>SMAAATFHWDDPLLLDQQLADDERMVRDAAHAYAQGKLAPRVTEAFRHETTDAAIFREMGEIGLLGPTIPEQYGGPGLDYVSYGLIAREVERVDSGYRSMMSVQSSLVMVPIFEFGSDAQKEKYLPKLATGEWIGCFGLTEPNHGSDPGSMVTRARKVPGGYSLSGSKMWITNSPIADVFVVWAKLDEDGRDEIRGFILEKGCKGLSAPAIHGKVGLRASITGEIVLDEAFVPEENILPHVKGLRGPFTCLNSARYGIAWGALGAAESCWHIARQYVLDRKQFGRPLAANQLIQKKLADMQTEITLGLQGVLRLGRMKDEGTA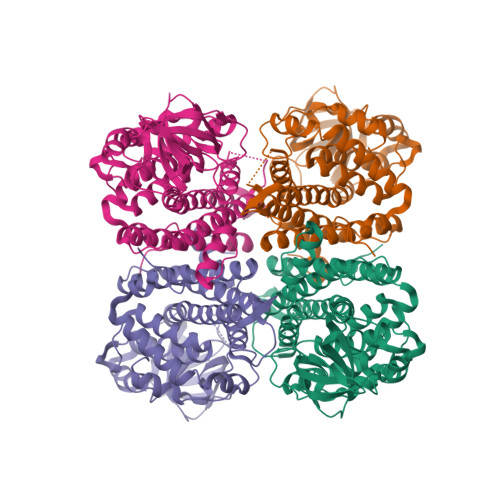AVEITSIMKRNSCGKALDIARLARDMLGGNGISDEFGVARHLVNLEVVNTYEGTHDIHALILGRAQTGIQAFF[4x]>MQKRADPPVALRHEGERLVVPAESPLRRTLAVAPATRETVAAPFNLPAMIEADPAKLVKVLPPLAGRIVSLNKQLGDEVKAGDVLFTIDSADLAQANSDAAKARAAMTMARRNLDRQRELDKSEIAAKRDFEQAQSDYDQAASESQRADARLAQLGAKGGGTLQAGGGHILAVRSPINGRVVDLNAATGAYWNDTTASLMTVADLSHVFVTANAQEKDLGHVYVGQSATVKFDAYDDPQPGKVRYVGQILDADTRTTKVRMVFDNPDGRLRPGMFAQATFLSQPHEGIVVPMSAIVQSGFYTRAFVEVAPWQFEP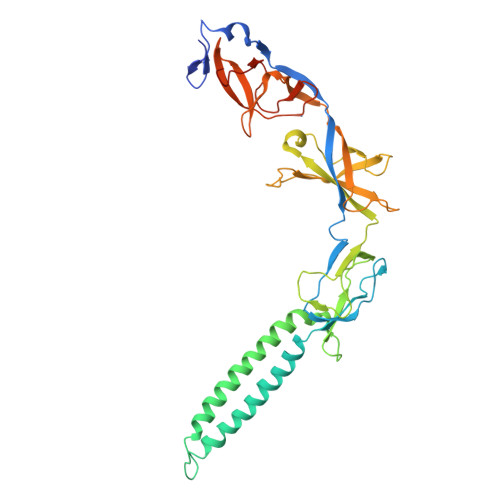RVIKLGAQIGDRMEVKSGLSAGDRVVVKEGVLLNDPDLLEVLFQ[2x]> SNAMTTMAETQTWQTVLGEEKQEPYFQEILDFVKKERKAGKIIYPPQKDIFNALKLTPYEAIKVVILGQDPYHGPNQAHGLAFSVRPGVPAPPSL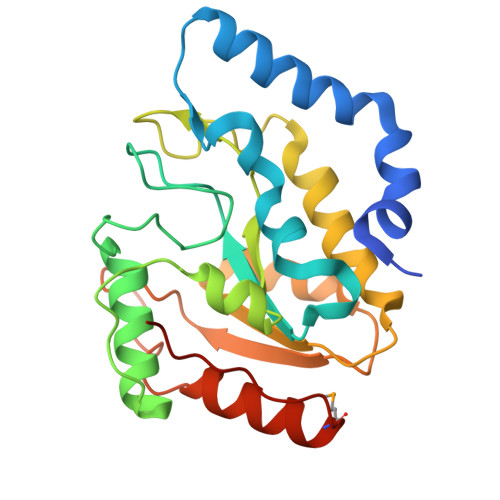QNIFKELHADLGVSIPSHGFLEKWAKQGVLLLNAALTVEAGKPQSHANIGWHRFTDKVIESLNDHPEGIVFLLWGSYAQKKSQLITNLRHRILKAPHPSPLSAARGFLGCRHFSKANQLLHEMGRGEIDWALDEKVS> SGPGCM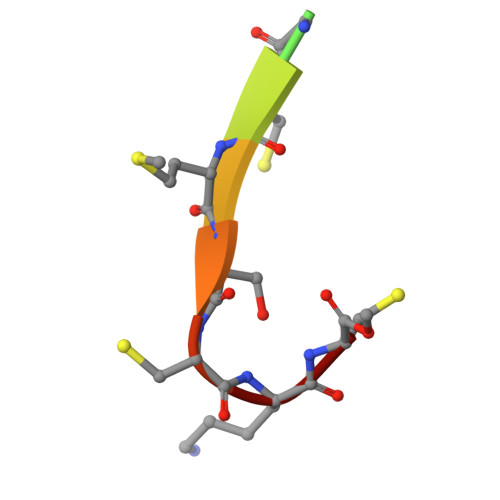SCKC>ALNSCPHVALLLSSGMGHLTPCLRFAATLVQHHCRVTIITNYPTVSVAESRAISLLLSDFPQITEKQFHLLPFDPSTANTTDPFFLRWEAIRRSAHLLNPLLSSISPPLSALVIDDSLVSSFVPVAANLDLPSYVLFTSSTRACSLEETFPAFVASKTNFDSIQLDDVIEIPGFSPVPVSSVPPTFLNLNHLFTTMLIQNGQSFRKANGILINTFEALEGGILPGINDKRAADGLPPYCSVGPLLPCKFEKTECSAPVKWLDDQPEGSVVYVSFGS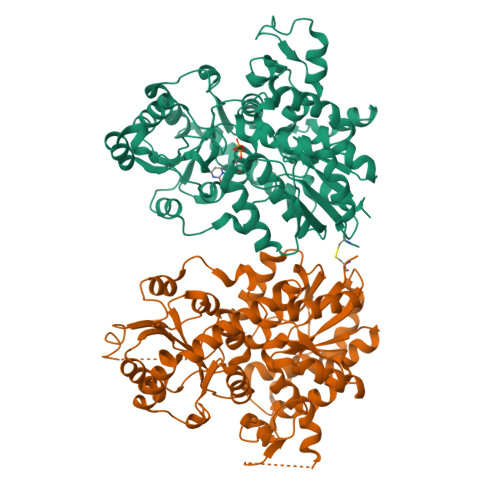RFALSSEQIKELGDGLIRSGCRFLWVVKCKKVDQEDEESLDELLGRDVLEKIKKYGFVIKNWVNQQEILDHRAVGGFVTHGGWNSSMEAVWHGVPMLVWPQFGDQKINAEVIERSGLGMWVKRWGWGTQQLVKGEEIGERIKDLMGNNPLRVRAKTLREEARKAIEVGGSSEKTLKELIENWK[2x]>SLEHHHHHHENLYFQGVGTRWAVLVAGSSGYGNYRHQADVCHAYQILRKGGLKEENIVVLMYDDIANHPLNPRPGTLINHPDGDDVYAGVPKDYTGSSVTAANFYAVLLGDQKAVKGGSGKVIASKPNDHIFVYYANHGGPGVLGMPNTPHIYAADFIETLKKKHASGTYKEMVIYVEAAESGSIFEGIMPKDLNIYVTTASNAQESSYGTYCPGMNPSPPSEYITCLGDLYSVAWMEDSETHNLKKETIKQQYHTVKMRTSNYNTYSGGSHVMEYGNNSIKSEKLYLYQGFDPATVNLPLNELPVKSKIGVVNQRDADLLFLWHMYRTSEDGSRKKDDTLKELTETTRHRKHLDASVELIATILFGPTMNVLNLVREPGLPLVDDWECLKSMVRVFEEHCGSLTQYGMKHMRAFANVCNNGVSKELMEEASTAACGGYSEARYTVHPSILGYSA[12x]

The plant cysteine proteases of the legumain family (C13 family, EC 3.4.22.34) have an important role in processing and maturation of seed storage proteins within the vacuole and, therefore, are also referred to as vacuolar processing enzymes (VPEs). Plant legumains are structurally related to the mammalian caspases and exhibit a strong substrate sequence preference for cleavage after asparagine and, to a lesser extent, aspartate residues. Seed type legumains like Arabidopsis thaliana legumain isoform β (AtLEGβ) play important functions in the processing and maturation of seed storage proteins within storage vacuoles. Structural analysis of plant legumains showed that they are synthesized as inactive zymogens composed of a caspase-like catalytic domain with AEP activity (AEP domain) and a C-terminal death domain-like prodomain (LSAM domain, legumain stabilization and activity modulation domain) that are connected by an activation peptide (AP) harboring the α6-helix.

To understand isoform-specific differences between different AtLEGs, we determined the crystal structure of seed-type proAtLEGβ to a resolution of 2.0 Å. The asymmetric unit of the tetragonal space group contained 12 independent molecules. Like isoform γ, proAtLEGβ comprises an N-terminal caspase-like catalytic domain and a C-terminal legumain stabilization and activity modulation (LSAM) domain with death domain-like topology. Overall, the structure of proAtLEGβ closely resembles the structure of the homologous two-chain AtLEGγ indicated by a Cα root mean square deviation (RMSD) of 0.49 Å. Similarly, in the crystal structure of proAtLEGβ, we found all twelve independent protomers in the crystallographic asymmetric unit to engage in symmetric dimer contacts, which were mediated by LSAM–LSAM′ interactions. In contrast, the proAtLEGβ dimers in the crystal structure were predominantly mediated by the α7 helix. This interaction was formed around the symmetric H384β (H392γ) and further stabilized by one symmetric salt bridge (E390β–K383β′) as well as by a hydrophobic contact of the α7 C-terminal LFG motif (396β-398β) with W355β′ centered in the α6 helix. However, modeling a proAtLEGγ-like dimer uncovered repulsive charge densities of α7-α7′ helix contact residues in AtLEGβ (R380–R380′, K373–K383′, and D369–D386′) that will prohibit this γ-mode of dimerization. Together, these findings suggest that the observed β-dimer is weak and probably only transient in solution. Comparing the crystal structure of proAtLEGβ with YVAD-cmk-inhibited AtLEGγ, we found that the AP binds to the nonprime substrate binding sites in a substrate-like orientation, similar to what we previously observed in mammalian prolegumain. Gln346 is binding into the S1 pocket in an unproductive orientation and thereby preventing cleavage of the AP and further blocking substrate access to the active site.>MKAQGQQLEVTKISSKVWIHTSYKTYHGTVVPSHGLIVSTKEGAVLIDTGWGKEPTEELLTWIKTNLKQPVKVCVPTHWHDDKLGGMEAVQRQGVPVVTSELTAILAAENSKGTPDVTFATDTTFAIG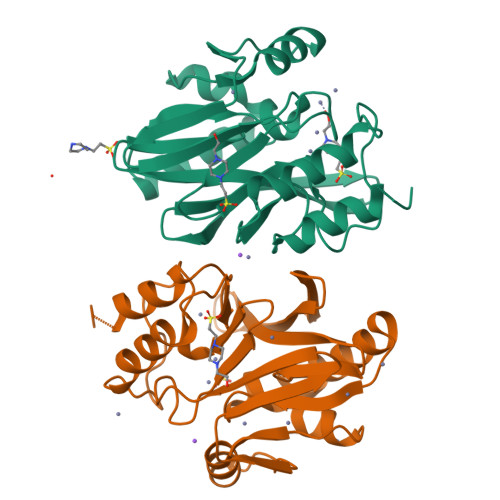GQQLEVYFPGGGHTADNVVVYLPQQKILFGGCLVKDLQAKNLGNTADADLKSWPLAIQRLQQRYPKAKVVVPSHGPWGDQSLLSHTLSLLQNQKQQNQ[2x]>[2x]MDTNQKLSIAVFALGCFWGPDAQFGSIKGVVSTRVGYAGGTTNNPSY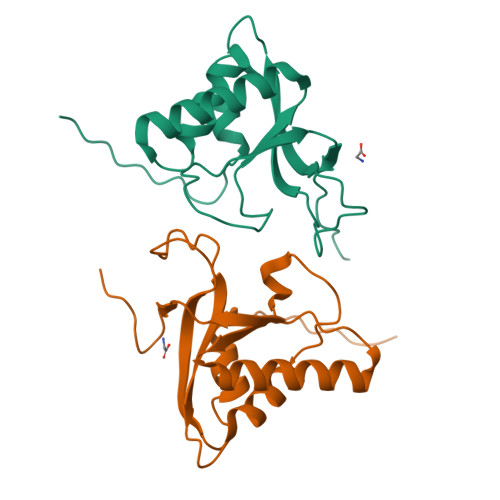YNLGDHSESIEIQYDANVITYGELLNIFWNLHNPVYETTNRQYMSRIFYLDDGQKSEALEMKRQIEAANGEKIYTEIVPLENFYLAEGYHQKYYLQN> MFKIVYPNAKDFFSFINSITNVTDSIILNFTEDGIFSRHLTEDKVLMAIMRIPKDVLSEYSIDSPTSVKLDVSSVKKILSKASSKKATIELTETDSGLKIIIRDEKSGAKSTIYIKAEKGQVEQLTEPKVNLAVNFTTDESVLNVIAADVTLVGEEMRISTEEDKIKIEAGEEGKR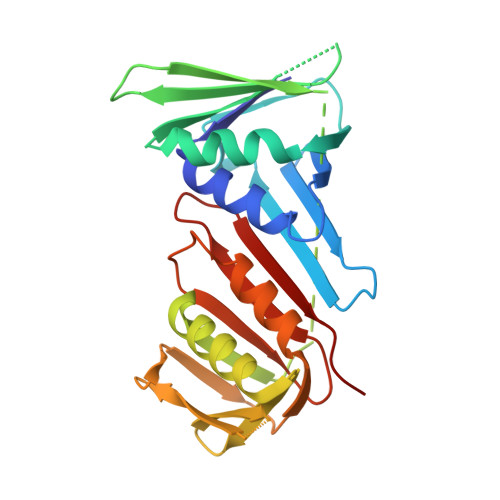YVAFLMKDKPLKELSIDTSASSSYSAEMFKDAVKGLRGFSAPTMVSFGENLPMKIDVEAVSGGHMIFWIAPRL>GSNSLMERIHEQIKKGELALFYLQEQINHFEEKPTKEMKDKIVAEMDTIIAMIDGVRGVLDRLMQRKDLDIFEQYNLEMAKKSGDILERDLKKEEARVKKIEV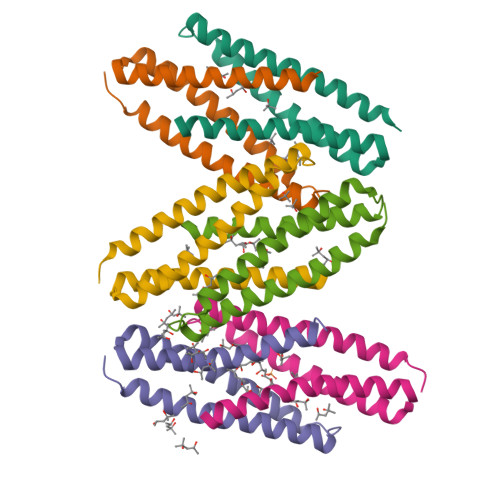[6x]> MSLSFTPLHTTSEAFIEKALPWLEDRYFHIAYLNPNGYTAYPQGAFRHYLAFGSEAAIHVSDATRVFETWNEIKKGYTNEWIFVFASYDGKNSVEQLHTSKEAGIAFAAATFFIPEHVWEIQPDGILIHKGSGSSLVTEIQHAEPSTPVQQSDIFVKQVVSKE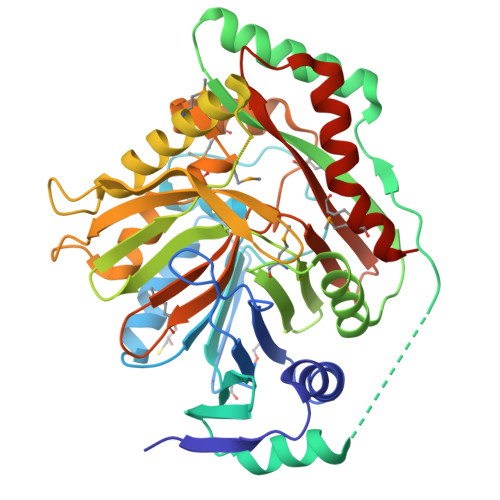SYFNAFDELQQIIAQGDAYEINYCIPFTAKGNISPAATYQRLNKKTPMPFSVYYKFNTEYILSASPERFIKKTGDTIISQPIKGTSKRGKSKAEDEMLKQQLGTSEKEQSENTMIVDLVRNDLSRTAVAGSVCVPELSGLYTFPNVHQLISTVQSTIDPACSSIDVIQQAFPMGSMTGAPKVNVMKFIDRIESMARGPFSGTVGYMDPHDNFDFNVLIRSIFYNSATQELFMEAGSAITSYAKAETEYEECLLKITPMIHILNNQEGHHHHHH>[4x]GSHMSLRYLRFLTAGESHGKGLTAILEGIPANLPLSEEEINHEL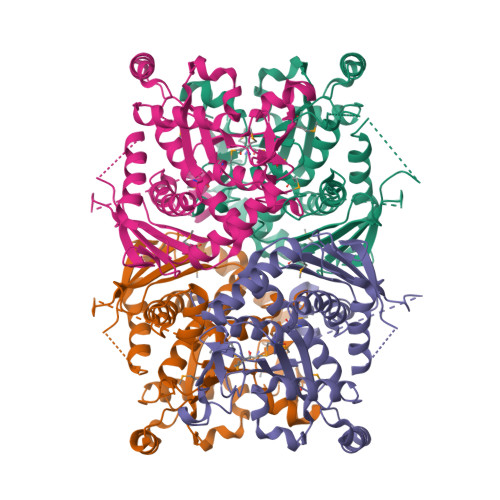RRRQRGYGRGGRMKIEKDTAEILSGVRFGKTLGSPIALFIRNRDWENWKEKMAIEGEPSPSVVPFTRPRPGHADLSGGIKYNQRDLRNILERASARETAARVAVGAVCKKFLSEFGIKIGSFVVSIGQKEVEELKDKSYFANPEKLLSYHEKAEDSELRIPFPEKDEEFKTYIDEVKEKGESLGGVFEVFALNVPPGLGSHIQWDRRIDGRIAQAMMSIQAIKGVEIGLGFEAARRFGSQVHDEIGWSEGKGYFRHSNNLGGTEGGITNGMPIVVRVAMKPIPTLKNPLRSVDIETKEEMKAGKERTDIVAVPAASVVGEAMLAIVLADALLEKLGGDFMEEVKKRFEDYVNHVKSF> MTVSFQEIHPIEIDAQWPRQPFYGFSLDSRKVETGQIFIALTSYSQPEKTRTFAEAALANGALAVISETELGVANEWVCPDVRQRMGEWQKRYLQQADVVKPLRIIAVTGTNGKTTISRLIAELISSQQQRCAVMGTTGNGILPNLTPSTHTTLDALQLQNALHDYAKQGATFASLEASSHGLEQGRLNGCDIEIAVYSNLSRDHLDYHGTLEAYAEAKARLFQFNSLKVAVINLDDAHADLMIKSAQNNPAQPKILTYSLTQNTADYYIADLDYSLAGATFNLVSQQGSFAVESPLLGHFNVENLIAALIAAEQAGFDLQALVDFVPKLIGAPGRMQVIRDDERLFVVDYAHTPDALIQVLKTLKRHVSNQLWAVFGCGGDRDRGKRPLMTQAALDGANPVILTSDNPRTEDPEQIFADMKQGIDFSGHRMHEIHDRREAIKFVAEQAQAGDIV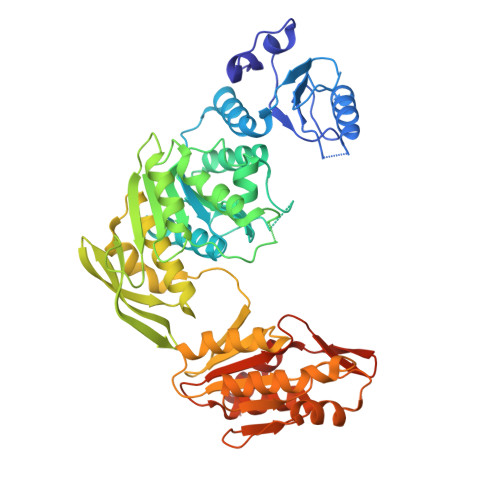VIAGKGHENYQEINGVRHWFDDVVEVRSAIDAQHHTVDAAYPAQ> DRVRSI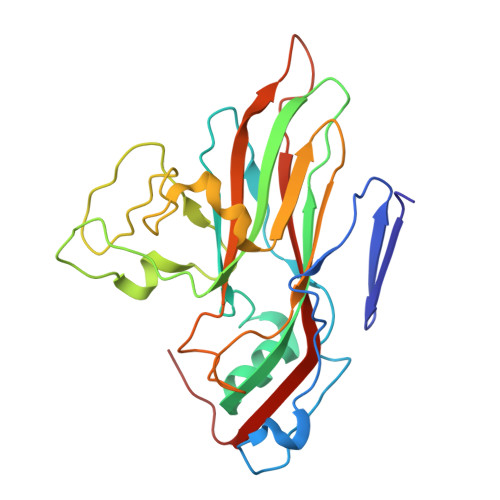TLGNSTITTQESANVVVAYGRWPEYLKDNEATAEDQPTQPDVATCRFYTLESVTWERDSPGWWWKFPDALKDMGLFGQNMYYHYLGRAGYTIHVQCNASKFHQGCLMVVCVPEAEMGCSQVDGTVNEHSLSEGETAKKFASTSTNGTNTVQSIVTNAGMGVGVGNLTIFPHQWINLRTNNCATIVMPYINNVPMDNMFRHHNFTLMIIPFVPLDYSSDSSTYVPITVTVAPMCAEYNGLRLATSL[FeFe]-hydrogenases represent one of natures’ most effective classes of redox enzymes catalyzing the reversible reduction of protons to dihydrogen (H2) at turnover frequencies of up to 9000 s-11–3. With their low catalytic over-potential, [FeFe]-hydrogenases represent excellent models for a regenerative and likewise economically feasible H2 production. Their active center (“H-cluster”) can be structured into a standard [4Fe-4S]-cluster ([4Fe]H) and a diiron site ([2Fe]H). Theoretical studies suggest that the most probable PT pathway comprises of strictly conserved residues E282, S319, E279, and C299 (from surface to H-cluster, numbering corresponds to CpI), including two protein-bound water molecules (Wat826, Wat1120 4XDC19, chain B) located between E279 and C29915,16,20. In this study, site-directed mutagenesis (SDM) is used to investigate the PT pathway of two [FeFe]-hydrogenases, namely CpI and HydA1, which represent the largest (M3) and smallest (M1) type of monomeric [FeFe]-hydrogenases, respectively.

Corresponding to earlier crystal structure data, for all CpI variants a space group of P1 21 1 was observed with two copies in the asymmetric unit cell (chain A and B). According to their close inter-residue distance of 2.8 Å, R286CpI may function as a salt bridge partner of deprotonated E282CpI and thus could be involved in the PT mechanism. R286CpI is further part of an extensive hydrogen-bonding network, which includes the carboxyl group of E282CpI, histidine residues H565CpI and H569CpI, and surface-bound H2O molecules. In case of variant R286A significantly fewer water molecules are observed in the same region. We therefore assume that the loss of the guanidine group in R286A destabilizes the network of proton-accepting/donating surface-bound H2O molecules near the entrance to the PT pathway. However, as the essential chain of PT pathway residues is not directly affected, the influence of this exchange on catalytic activity is comparatively weak. Variants E282DCpI, C299DCpI, R286ACpI, and E282ACpI were only mildly affected and showed residual activities between 30 and 90%.

>[2x]MKTIIINGVQFNTDEDTTILKFARDNNIDISALCFLNNCNNDINKCEICTVEVEGTGLVTACDTLIEDGMIINTNSDAVNEKIKSRISQLLDIHEFKCGPCNRRENCEFLKLVIKYKARASKPFLPKDKTEYVDERSKSLTVDRTKCLLCGRCVNACGKNTETYAMKFLNKNGKTIIGAEDEKCFDDTNCLLCGQCIIACPVAALSEKSHMDRVKNALNAPEKHVIVAMAPSVRASIGELFNMGFGVDVTGKIYTALRQLGFDKIFDINFGADMTIMEEATELVQAIENNGPFPMFTSCCPGWVRQAENYYPELLNNLSSAKSPQQIFGTASKTYYPSISGLDPKNVFTVTVMPCTSKKFEADRPQMEKDGLRDIDAVITTRELAKMIKDAKIPFAKLEDSEADPAMGEYSGAGAIFGATGGVMEAALRSAKDFAENAELEDIEYKQVRGLNGIKEAEVEINNNKYNVAVINGASNLFKFMKSGMINEKQYHFIEVMACHGGCVNGGGQPHVNPKDLEKVDIKKVRASVLYNQDEHLSKRKSHENTALVKMYQNYFGKPGEGRAHEILHFKYKKSAWSHPQFEK>[2x]GHMPNIPPPFTAPYAPDDAEIAARLLPASHLSPPQEARIHRTATRLIEAIRKRDDRLGGVEDMLREFALSTKEGLALMVLAEALLRVPDARTADQFIEDKLGEGDFIHHETKSTAFLVNASAWALGLSARVIQPGETPDGTIGRLVKRLGAPAVRTATRQAMRLMGNHFVLGETIEQALERGKPRSGQKTRYSFDMLGEGARTAADARRYFDAYASAIETIGKAAGNHALPDRPGISVKLSALHPRFEAISRARVMVELVPQLLDLAQRAKAHDLNFTVDAEEADRLELSLD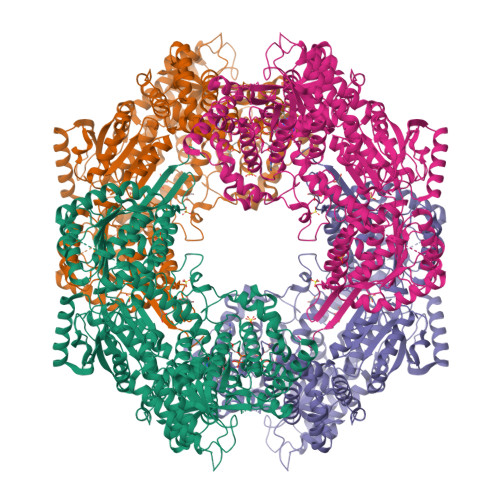VIAATLADPSLKGWDGFGLAIQAYQKRASAVIDYVDALARAHDRKLMVRLVKGAYWDTEIKRAQERGLDGYPVFTRKAMTDLNYVACASKLLALRPRIFPQFATHNALTVATVLEMAEGSSGFEFQRLHGMGEALYEQLAKDHADIAYRTYAPVGSHRDLLAYLVRRLLENGANSSFVAQAADYRVPVPALLQRPADAIVRPQAAAHPRIPLPCDLFAPERRNSRGVEFGARTALDQLLTDVKAETGDLKPIADATPDQAHAAVAAARAGFAGWSRTPAGIRAAALEQAAHLLESRSAHFIALLQREGGKTLDDALSELREAADFCRYYAAQGRKLFGSETAMPGPTGESNALTMRGRGVFVAISPWNFPLAIFLGQVTAALMAGNSVVAKPAEQTPRIAREAVALLHEAGIPKSALYLVTGDGRIGAALTAHPDIAGVVFTGSTEVARSINRALAAKDGPIVPLIAETGGINAMIADATALPEQVAYDVVTSAFRSAGQRCSALRLLFVQEDVADRMIEMVAGAARELKIGDPSDVATHVGPVIDVEAKQRLDAHIARMKTEARLHFAGPAPEGCFVAPHIFELTEAGQLTEEVFGPILHVVRYRPENLERVLRAIERTGYGLTLGVHSRIDDSIEAIIDRVQVGNIYVNRNMIGAVVGVQPFGGNGLSGTGPKAGGPHYLARFATEQTVTINTAAAGGNAALLAGEE In the ethanologenic bacterium Zymomonas mobilis ZM4, the gene ZMO0922 encodes a 148 amino acid polypeptide, which has been annotated as a putative ASCH domain-containing protein (ZmASCH) that belongs to family 23. Here, we report the three-dimensional crystal structure of ZmASCH which confirms the fold of a central β-barrel core and reveals a positively-charged cleft with a pocket on the surface. In vitro assays showed that ZmASCH bound nucleic acids and possessed cleavage activity specifically towards single-stranded RNAs. The weak nuclease activity of ZmASCH depended on magnesium ions and the protein appeared to prefer the consecutive pyrimidine-adenine dinucleotides for its cleavage activity.

Thr49, Arg50, Lys53, and Gln127 directly interact with atoms of the phosphate backbone, while Tyr47 forms an interaction with the phosphate moiety between the −1 and +1 nucleotides through the intervening water molecules. However, removal of the side-chain hydroxyl group in Tyr47 (Y47F) substantially decreased the DNA- and RNA-binding activity of the protein. In addition, this Y47F mutant also possessed decreased RNA-hydrolytic activity. Mutations of the two independent residues at the positions of 47 and 128 did not make a noticeable structural change. There are two and four protein molecules in the asymmetric unit of the trigonal and monoclinic crystal forms, respectively. The conformations of individual monomers are in excellent agreement, and all monomers superimpose with RMSD values of less than 0.3 Å, with the largest deviations in the loops between strands β2 and β3 and helices α4 and α5.

>[4x]AMTDIPDRKEAVISLWPEFAKAIVSGKKTVEFRRRIPLPALSARIWIFATRPVKSVIGFAYLEAIVQGDVNTLWSRYGREAFLSEQQYRDYFEGTEKATAFLLRDHQPIRPINLDQLKEIRANFQPPQSLTWLRKEETQKLVSLTSQVE> MAITAYSQQTRGLLGCIITSLTGRDKNQVEGEVQVVSTATQSFLATCVNGVCWTVYHGAGSKTLAGPKGPITQMYTNVDQDLVGWQAP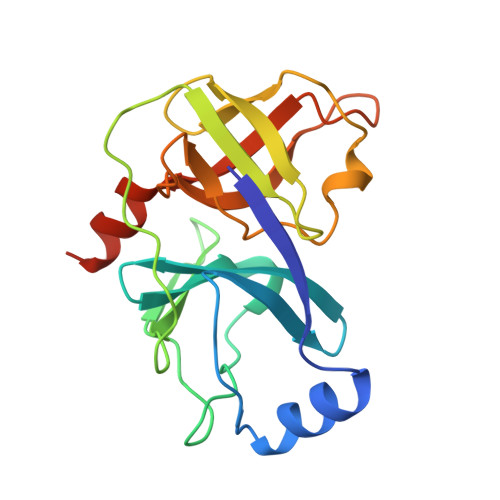PGARSLTPCTCGSSDLYLVTRHADVIPVRRRGDSRGSLLSPRPVSYLKGSSGGPLLCPSGHAVGIFRAAVCTRGVAKAVDFVPVESMETTMRMRKKKK> MHHHHHHSSGMGEKLELRLKSPVGAEPAVYPWPLPVYDKHHDAAHEIIETIRWVCEEIPDLKLAMENYVLIDYDTKSFESMQRLCDKYNRAIDSIHQLWKGTTQPMKLNTRPSTGLLRHILQQVYNHSVTDPEKLNNYEPFSPEVYGETSFDLVAQMIDEIKMTDDDLFVDLGSGVGQVVLQVAAATNCKHHYGVEKADIPAKYAETMDREFRKWMKWYGKKHAEYTLERGDFLSEEWRERIANTSVIFVNNFAFGPEVDHQLKERFANMKEGGRIVSSKPFAPLNFRINSRNLSDIGTIMRVVELSPLKGSVSWTGKPVSYYLHTIDRTILENYFSSLKNPKLREEQEAARRRQQRESKSNAATPTKGPEGKVAGPADAPMDSGAEEEKAGAATVKKPSP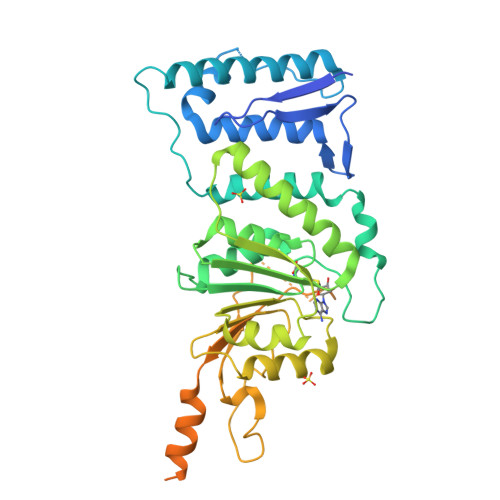SKARKKKLNKKGRKMAGRKRGRPKK>VSPPPPIADEPLTVNTGIYLIECYSLDDKAETFKVNAFLSLSWKDRRLAFDPVRSGVRVKTYEPEAIWIPEIRFVNVENARDADVVDISVSPDGTVQYLERFSARVLSPLDFRRYPFDSQTLHIYLIVRSVDTRNIVLAVDLEKVGKNDDVFLTGWDIESFTAVVKPANFALEDRLESKLDYQLRISRQYFSYIPNIILPMLFILFISWTAFWSTSYEANVTLVVSTLIAHIAFNILVETNLPKTPYMTYTGAIIFMIYLFYFVAVIEVTVQHYLKVESQPARAASITRASRIAFPVVFLLANI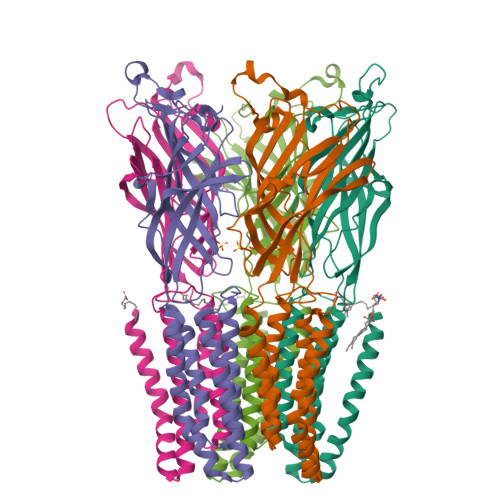ILAFLFF[5x]>ALPDLKIEKLEEGVFVHTSFEEVNGWGVVTKHGLVVLVNTDAYLIDTPFTATDTEKLVNWFVERGYEIKGTISSHFHSDSTGGIEWLNSQSIPTYASELTNELLKKSGKVQAKYSFSEVSYWLVKNKIEVFYPGPGHTQDNLVVWLPESKILFGGCFIKPHGLGN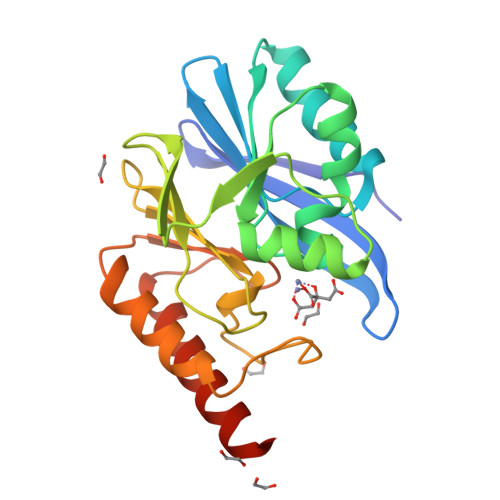LGDANLEAWPKSAKILMSKYGKAKLVVSSHSEKGDASLMKRTWEQALKGLKESKKTSSPSN[3x]>[2x]MKSEPLSYLGKDGGPWEIFTEQVDRVVPYLGRLAPLAESLKRPKRVLIVDVPVRLDDGSVAYFEGYRVHHNTARGPAKGGVRYHPEVTLSEVMALAGWMTIKNAAVGLPYGGGKGGIRVDPRKLSPGELERLTRRYTSEIGILLGPDRDIPAPDVNTGEREMAWMMDTYSMNVGRTVPGVVTGKPIALGGSLGRRDATGRGVFITAAAAAEKIGLQVEGARVAIQGFGNVGNAAARAFHDHGARVVAVQDHTGTVYNEAGIDPYDLLRHVQEFGGVRGYPKAEPLPAADFWGLPVEFLVPAALEKQITEQNAWRIRARIVAEGANGPTTPAADDILLEKG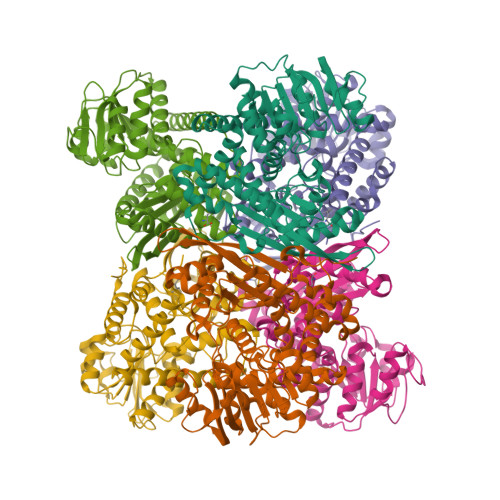VLVVPDVIANAGGVTVSYFEWVQDFNSYFWTEEEINARLERVLRNAFEAVWQVAQEKKIPLRTAAYVVAATRVLEARALRGLYP;>MPLKAYRPPEDPGLWDTYLEWLERALKVAGVHPTTLEYLAHPKRLVTLSLPVVMDDGKVRIFQGYRVVHDIARGPAKGGVRLDPGVTLGQTAGLAAWMTLKAAVYDLPFGGAAGGIAVDPKGLSPQELERLVRRYTAELVGLIGPDSDILGPDLGADQQVMAWIMDTYSMTVGSTVPGVVTGKPHALGGSEGRDDAAGLGALLVLEALAKRRGLDLRGARVVVQGLGQVGAAVALHAERLGMRVVAVATSMGGMYAPEGLDVAEVLSAYEATGSLPRLDLAPEEVFGLEAEVLVLAAREGALDGDRARQVQAQAVVEVANFGLNPEAEAYLLGKGALVVPDLLSGGGGLLASYLEWVQDLNMFFWSPEEVRERFETRVARVVDAVCRRAERGGLDLRMGALALALERLDEATRLRGVYP[4x]>[3x]MDFSRNLYDIGEQLDSEDLASLKFLSLDYIPQRKQEPIKDALMLFQRLQEKRMLEESNLSFLKELLFRINRLDLLITYLNTRKEEMERELQTPGRAQISAYRVMLYQISEEVSRSELRSFKGGLQEEIS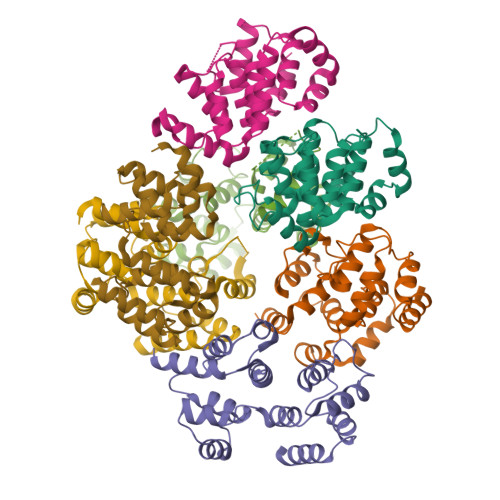KCKLDDDMNLLDIFIEMEKRVILGEGKLDILKRVCAQINKSLLKIINDYEEFSKERSSSLEGSPDEFSNGEELCGVMTISDSPREQDSESQTLDKVYQMKSKPRGYCLIINNHNFAKAREKVPKLHSIRDRNGTHLDAGALTTTFEELHFEIKPHDDCTVEQIYEILKIYQLMDHSNMDCFICCILSHGDKGIIYGTDGQEAPIYELTSQFTGLKCPSLAGKPKVFFIQAAQGDNYQKGIPVETASEEQPYLEMALSSPQTRYIPDEADFLLGMATVNNCVSYRNPAEGTWYIQSLCQSLRERCPRGDDILTILTEVNYEVSNKDDKKNMGKQMPQPTFTLRKKLVFPSD;>[4x]MSAEVIHQVEEALDTDEKEMLLFLCRDVAIDVVPPNVRDLLDILRERGKLSVGDLAELLYRVRRFDLLKRILKMDRKAVETHLLRNPHLVSDYRVLMAEIGEDLDKSDVSSLIFLMKDYMGRGKISKEKSFLDLVVELEKLNLVAPDQLDLLEKCLKNIHRIDLKTKIQKYKQSVQGAGTS> MSEIGTGFPFDPHYVEVLGERMHYVDVGPRDGTPVLFLHGNPTSSYLWRNIIPHVAPSHRCIAPDLIGMGKSDKPDLDYFFDDHVRYLDAFIEALGLEEVVLVIHDWGSALGFHWAKRNPERVKGIACMEFIRPIPTWDEWPEFARETFQAFRTADVGRELIIDQNAFIEGVLPKCVVRPLTEVEMDHYREPFLKPVDREP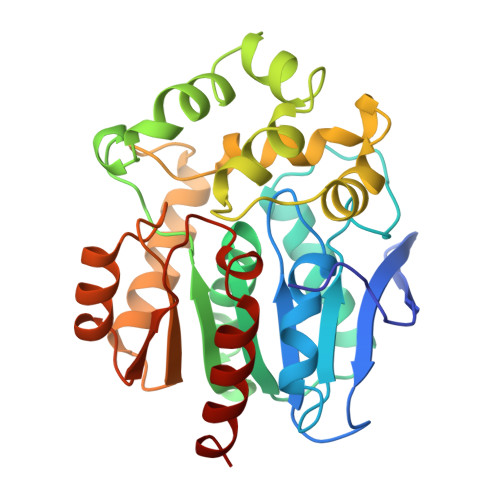LWRFPNEIPIAGEPANIVALVEAYMNWLHQSPVPKLLFWGTPGVLIPPAEAARLAESLPNCKTVDIGPGLHYLQEDNPDLIGSEIARWLPGLA>GPSNAEYSKVPDVEGQDKQKAIDNVSAKSLEPVTIGSGTQIKAQSIKAGNKVLPHSKVLLLTDGDLTMPDMSGWTKEDVIAFENLTNIKVNLKGSGFVSHQSISKGQKLTEKDKIDVEFSSENVDSNSTNNSDSNSDDKKKS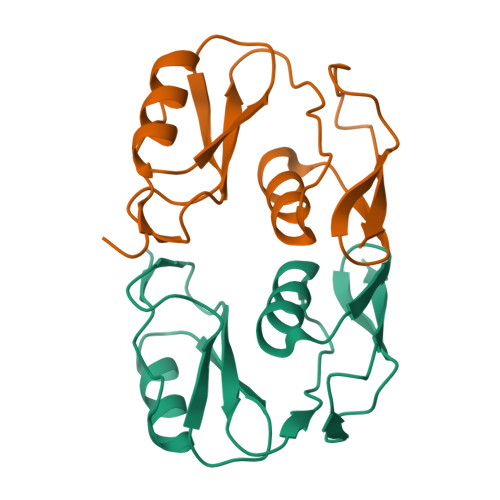DSKTDKDKSD[2x]> MRETHLRSILHTIPDAMIVIDGHGIIQLFSTAAERLFGWSELEAIGQNVNILMPEPDRSRHDSYISRYRTTSDPHIIGIGAIVT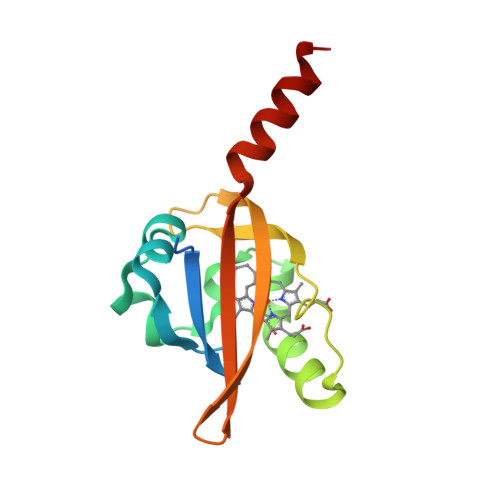GKRRDGTTFPMHLSIGEMQSGGEPYFTGFVRDLTEHQQTQARLQELQ> MRLKNLTFIIILIISGELYAEEKPCGFPHVENGRIAQYYYTFKSFYFPMSIDKKLSFFCLAGYTTESGRQEEQTTCTTEGWSPEPRCFKKCTKPDLSNGYISDVKLLYKIQENMRYGCASGYKTTGGKDEEVVQCLSDGWSSQPTCRKEHETCLAPELYNGNYSTTQKTFKVKDKVQYECATGYYTAGGKKTEEVECLTYGWSLTPKCTKLKCSSLRLIENGYFHPVKQTYEEGDVVQFFCHENYYLSGSDLIQCYNFGWYPESPVCEGRRNRCPPPPLPINSKIQTHSTTYRHGEIVHIECELNFEIHGSAEIRCEDGKWTEPPKCIEGQEKVACEEPPFIENGAANLHSKIYYNGDKVTY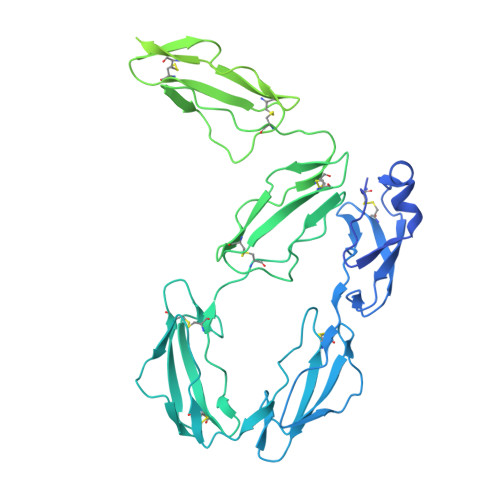ACKSGYLLHGSNEITCNRGKWTLPPECVENNENCKHPPVVMNGAVADGILASYATGSSVEYRCNEYYLLRGSKISRCEQGKWSSPPVCLEPCTVNVDYMNRNNIEMKWKYEGKVLHGDLIDFVCKQGYDLSPLTPLSELSVQCNRGEVKYPLCTRKESKGMCTSPPLIKHGVIISSTVDTYENGSSVEYRCFDHHFLEGSREAYCLDGMWTTPPLCLEPCTLSFTEMEKNNLLLKWDFDNRPHILHGEYIEFICRGDTYPAELYITGSILRMQCDRGQLKYPRCIPRQSTLSYQEPLRT> METSDIQIFYQEDPECQNLSENSCPPSEVSDTNLYSPFKPRNYQLELALPAMKGKNTIICAPTGCGKTFVSLLICEHHLKKFPQGQKGKVVFFANQIPVYEQQKSVFSKYFERHGYRVTGISGATAENVPVEQIVENNDIIILTPQILVNNLKKGTIPSLSIFTLMIFDECHNTSKQHPYNMIMFNYLDQKLGGSSGPLPQVIGLTASVGVGDAKNTDEALDYICKLCASLDASVIATVKHNLEELEQVVYKPQKFFRKVESRISDKFKYIIAQLMRDTESLAKRICKDLENLSQIQNREFGTQKYEQWIVTVQKACMVFQMPDKDEESRICKALFLYTSHLRKYNDALIISEHARMKDALDYLKDFFSNVRAAGFDEIEQDLTQRFEEKLQELESVSRDPSNENPKLEDLCFILQEEYHLNPETITILFVKTRALVDALKNWIEGNPKLSFLKPGILTGRGKTNQNTGMTLPAQKCILDAFKASGDHNILIATSVADEGIDIAQCNLVILYEYVGNVIKMIQTRGRGRARGSKCFLLTSNAGVIEKEQINMYKEKMMNDSILRLQTWDEAVFREKILHIQTHEKFIRDSQEKPKPVPDKENKKLLCRKCKALACYTADVRVIEECHYTVLGDAFKECFVSRPHPKPKQFSSFEKRAKIFCARQNCSHDWGIHVKYKTFEIPVIKIESFVVEDIATG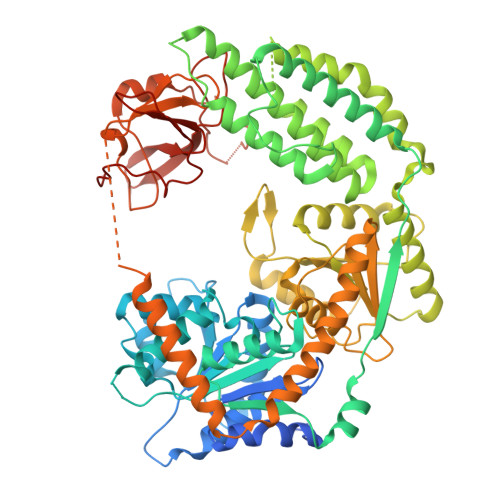VQTLYSKWKDFHFEKIPFDPAEMSK> GAMGSSTEDASQYYCDKNDNGDSYLVLIRITPDEDGKFGFNLKGGVDQKMPLVVSRINPESPADTCIPKLNEGDQIVLI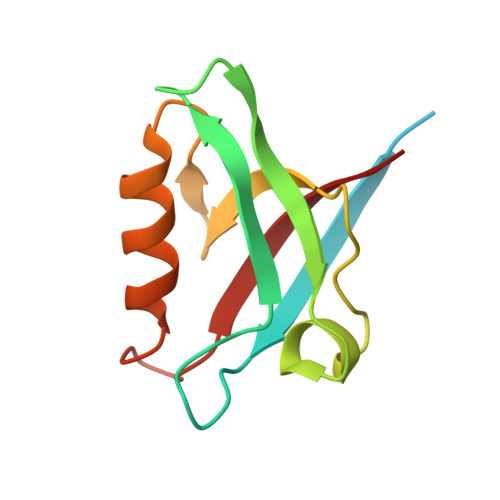NGRDISEHTHDQVVMFIKASRESHSRELALVIRRR GMP synthetase (EC 6.3.5.2) is a glutamine amidotransferase that catalyzes the final step of de novo GMP biosynthesis, whereby it converts xanthosine 5′-monophosphate (XMP) to guanosine 5′-monophosphate (GMP). GMPS is made up of two domains, one being a glutaminase (GATase) domain that catalyzes the hydrolysis of the amino acid glutamine to glutamate and ammonia. The generated ammonia is used by the ATP pyrophosphatase (ATPPase) domain to catalyze the amination of XMP to form the end product, GMP. Functional GMPS dimers associate through the dimerization domain.

Here, we present novel findings that add further insight into the functioning of this enzyme with a structure of a variant in which not only the catalytic Cys89 was mutated, but also Cys113, which was earlier shown to form a disulfide bridge with Cys377 in the PfGMPS_C89A/Gln complex. The crystal structure of this mutant solved by molecular replacement was determined to a 2.8 Å resolution. The GATase domain of the double mutant (PfGMPS_C89A_C113A) is rotated by ~170° and translated ~1.5 Å compared to the native structure and when holding the ATPPase domain fixed. If compared with the structure of the single mutant, the GATase domain is rotated by ~120° and translated ~4 Å, again when holding the ATPPase domain fixed. The electron density of this double mutant revealed a crystal structure that is not only more collapsed than the wild-type and single mutant enzymes described earlier but also significantly less structured, resulting in bad geometry, as can be observed from the Ramachandran parameters. Destructuring is particularly important in the ATPPase domain, and to our surprise, the observed structure of this double mutant is a monomeric enzyme. The monomeric nature of the double mutant in solution was confirmed by Small Angle X-ray Scattering studies, as opposed to the solution dimers observed earlier for the PfGMPSwt and PfGMPS_C89A enzymes and confirmed herein. Unequivocally, the double mutant is no longer able to form this disulfide bridge, resulting in an enzyme that, in principle, can continue its rotation. By all means, besides presenting an enzyme with a partly destroyed substrate binding pocket in the ATPPase domain, in PfGMPS_C89A_C113A, the interactions that are critical for ensuring correct ammonia channeling from the GATase domain to the ATPPase domain are modified. Hence, mutation of Cys113 to an alanine precludes the enzyme from resting in a conformation in which ammonia is in the correct position for attacking the AMP-XMP intermediate, as observed earlier in the 85° rotated enzyme.

> MRGSHHHHHHGSMAEGEEYDKILVLNFGSQYFHLIVKRLNNIKIFSETKDYGVELKDIKDMNIKGVILSGGPYSVTEAGSPHLKKEVFEYFLEKKIPIFGIAYGMQEIAVQMNGEVKKSKTSEYGATDVNILRNDNINNITYCRNFGDSSSAMDLYSNYKLMNETCCLFENIKSDITTVWMNHNDEVTKIPENFYLVSSSENCLICSIYNKEYNIYGVQYHPEVYESLDGELMFYNFAYNICKCKKQFDPIRYHELELKNIEKYKHDHYVIAAMSGGIDSTVAAAYTHKIFKERFFGIFIDNGLLRKNEAENVYTFLKSTFPDMNITKIDASENFLSNLQGVTDPEQKRKIIGKLFIEEFEKAVNNIDIDINKTFLLQGTLYPDIIESKCSKNLSDTIKTHHNVGGLPKNLKFKLFEPFKYLFKDDVKTLSRELNLPEEITNRHPFPGPGLAIRVIGEINKHKLNILREVDDIFINDLKQYGLYNQISQAFAVLLSSKSVGVRGDARSYDYVCVLRAVKTSSFMTANWYQIPYDILDKITTRILSEVKGVNRILYDVSSKPPATIEFE The centromere binding factor 3 (CBF3) complex binds the third centromere DNA element in organisms with point centromeres, such as S. cerevisiae. It is an essential complex for assembly of the kinetochore in these organisms, as it facilitates genetic centromere specification and allows association of all other kinetochore components. CBF3 comprises two homodimers, of Cep3 and Ndc10, and a Ctf13-Skp1 heterodimer. Cep3 provides sequence specificity through binuclear zinc-cluster (Zn2Cys6) domains homologous to those found in GAL4-like fungal transcription factors (Lechner, 1994, MacPherson et al., 2006).

Full-length Cep3 rendered CBF3CC relatively unstable, but the complex with an N-terminally truncated Cep3, in which the Zn2Cys6 domains were missing, yielded a 220 kDa complex (CBF3CCΔN) that was purified to homogeneity and was suitable for cryo-EM studies. After refinement, the final map was calculated from 187,606 particles, with a resolution of 3.7 Å judged using the Fourier shell correlation (FSC) gold standard method. Secondary structure details and side chains were clearly visible throughout the CBF3CCΔN map, enabling an atomic model for the core complex to be built and refined. The 2.5 Å crystal structure of the Cep3ΔN homodimer was fit in the map as a rigid body, and this structure is essentially unchanged after refinement with a final Cα RSMD of 1.1 Å. The most striking secondary structural feature of this model is an eight-stranded parallel β sheet. This is part of a larger solenoid structure, corresponding to the predicted leucine-rich repeat (LRR) fold of Ctf13, and comprises eight LRR motifs, rather than seven LRRs identified previously (Leber et al., 2018). The remaining flanking density is an α-β subdomain that decorates the C-terminal end of the Ctf13 LRR, formed by insertions within the last 3 LRRs of Ctf13. This subdomain contacts and stabilizes a typically disordered acidic loop of Skp1 such that the Skp1-Ctf13 heterodimer forms a toroidal structure in which both the N-terminal F box and the C-terminal α-β LRR-insertion domain of Ctf13 associate with either end of Skp1. The Ctf13-Skp1 heterodimer forms the left side of the horseshoe and makes extensive contacts with the base, formed by the “proximal” monomer of the Cep3 homodimer. The “distal” monomer of the Cep3 dimer forms the remaining side of the horseshoe. This arrangement positions the truncated Zn2Cys6 domains of (Cep3ΔN)2 at opposite ends of the channel created by the horseshoe. Ctf13 and Cep3 line the channel with basic residues that are strongly conserved between Saccharomycetaceae.

>[2x]MGGSSHHHHHHSSGLVPRGSHMKLITASSSKEYLPDLLLFWQNYEYWITNIGLYKTKQRDLTRTPANLDTDTEECMFWMNYLQKDQSFQLMNFAMENLGALYFGSIGDISELYLRVEQYWDRRADKNHSVDGKYWDALIWSVFTMCIYYMPVEKLAEIFSVYPLHEYLGSNKRLNWEDGMQLVMCQNFARCSLFQLKQCDFMAHPDIRLVQAYLILATTTFPYDEPLLANSLLTQCIHTFKNFHVDDFRPLLNDDPVESIAKVTLGRIFYRLCGCDYLQSGPRKPIALHTEVSSLLQHAAYLQDLPNVDVYREENSTEVLYWKIISLDRDLDQYLNKSSKPPLKTLDAIRRELDIFQYKVDSLEEDFRSNNSRFQKFIALFQISTVSWKLFKMYLIYYDTADSLLKVIHYSKVIISLIVNNFHAKSEFFNRHPMVMQTITRVVSFISFYQIFVESAAVKQLLVDLTELTANLPTIFGSKLDKLVYLTERLSKLKLLWDKVQLLDSGDSFYHPVFKILQNDIKIIELKNDEMFSLIKGLGSLVPLNKLRQESLLEEEDENNTEPSDFRTIVEEFQSEYNISDILS;> MGVTSNVVLVSGEGERFTVDKKIAERSLLLKNYLNDMHDSNLQNNSDSESDSDSETNHKSKDNNNGDDDDEDDDEIVMPVPNVRSSVLQKVIEWAEHHRDSNFPDEDDDDSRKSAPVDSWDREFLKVDQEMLYEIILAANYLNIKPLLDAGCKVVAEMIRGRSPEEIRRTFNIVNDFTPEEEAAIRRENEWAEDRGS;> MGPSFNPVRFLELPIDIRKEVYFHLDGNFCGAHPYPIDILYKSNDVELPGKPSYKRSKRSKKLLRYMYPVFATYLNIFEYSPQLIEKWLEYAFWLRYDCLVLDCFKVNHLYDGTLIDALEWTYLDNELRLAYFNKASMLEVWYTFKEYKKWVIDSVAFDELDLLNVSNIQFNIDNLTPQLVDKCLSILEQKDLFATIGEVQFGQDEEVGEEKDVDVSGANSDENSSPSSTIKNKKRSASKRSHSDNGNVGATHNQLTSISVIRTIRSMESMKSLRKITVRGEKLYELLINFHGFRDNPGKTISYIVKRRINEIRLSRMNQISRTGLADFTRWDNLQKLVLSRVAYIDLNSIVFPKNFKSLTMKRVSKIKWWNIEENILKELKVDKRTFKSLYIKEDDSKFTKFFNLRHTRIKELDKSEINQITYLRCQAIVWLSFRTLNHIKLQNVSEVFNNIIVPRALFDSKRVEIYRCEKISQVLVIGSRSGSENLYFQGSKRRWKKNFIAVSAANRFKKISSSGAL>MGHHHHHHHHEFIPSNTDYPGPHHFEVTFQQSSTAKFATWTYSPLLKKLYCQIAKTCPIQIKVSTPPPPGTAIRAMPVYKKAEHVTDVVKRCPNHELGRDFNEGQSAPASHLIRVEGNNLSQYVDDPVTGRQSVVVPYEPPQVGTEFTTILYNFMCNSSCVGGMNRRPILIIIT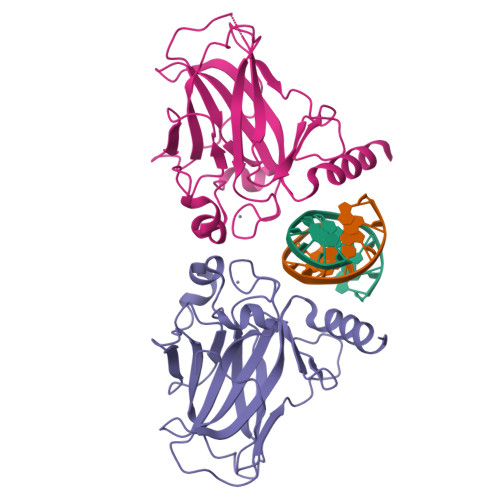LEMRDGQVLGRRSFEGRICACPGRDRKADEDHYREQ[2x]> QTKAEENKKPNILFIITDDHAYQTLGTGNNDSPVALPNFNKLGRQGMVFDRSYCANSLCGPSRACILTGRHSHMNGFVFNGQRPLDGSQPTYPKMLQKAGYQTGLFGKWHLESDPTGFDTWEIFPGQGSYYNPDFISLKPDGKRQTKRFPGYATDVVTDKSIQWLGNRDKNKPFLLVVGHKAPHRAWCPALRHLGKVDTSSMTPPANFHDD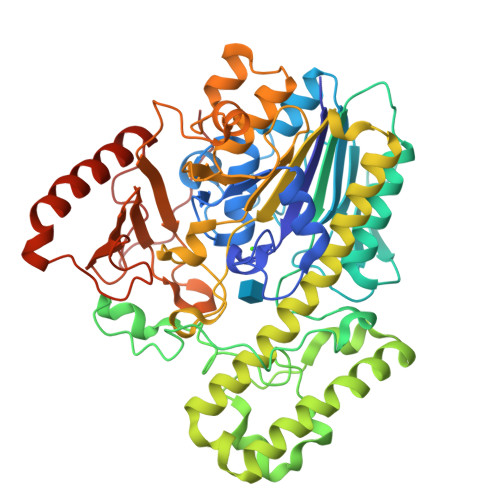YANRPEFLKKNQQTVANHMAIYSDLKVLKDQVPEEMRKSIVSPGYGWDLGELNRMTPEEKKTWTDYYAKRTKSLVDGMKSGKLKDPKAFAEWKWHAYMEDYLGCLLSVDDSIGRLMEYLDKEGIAKDTLVIYCGDQGFYMGEHGMYDKRWIFEESLRMPLIMRWPGKIPAGIRNNTMVQNIDYAPTIVSAAGADTPENMNTFQGVSLLPTAFTGKTPDNWRDAIYYCFYENPGEHNAPRHDGIRTDRYTLSYIWTSDEWMLFDMKKDPMQMKNVIDDPAYKTTVEQLKKRYHELRKTYKVPENSPGGKGTPIPKFDASW>[2x]MHHHHHHASENLYFQGAMVMGNQQVVSITGAGSGIG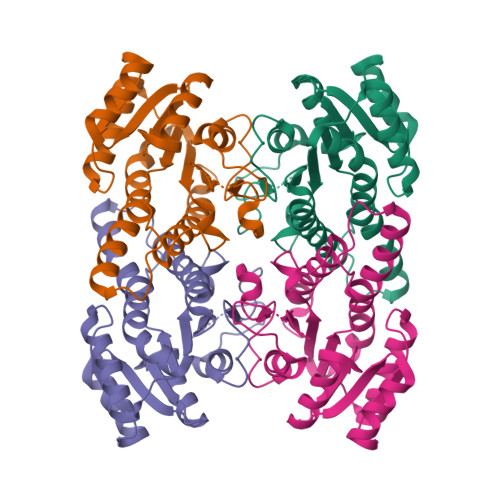LELVRSFKLAGYCVSALVRNEEQEALLCNEFKDALEIVVGDVRDHATNEKLIKQTIDRFGHLDCFIANAGIWDYMLNIEEPWEKISSSFDEIFDINVKSYFSGISAALPELKKTNGSVVMTASVSSHAVGGGGSCYIASKHAVLGMVKALAYELAPEIRVNAVSPGGTVTSLCGPASAGFDKMHMKDMPGIDDMIKGLTPLGFAAKPEDVVAPYLLLASRKQGKFITGTVISIDGGMALGRK>[2x]MRGSHHHHHHGLVPRGSMIRTMLQGKLHRVKVTHADLHYEG;>XCAIDQDFLDAAGILENEAIDIWNVTNGKRFSTYAIAAERGSRIISVNGAAAHCASVGDIVIIASFVTMPDEEARTWRP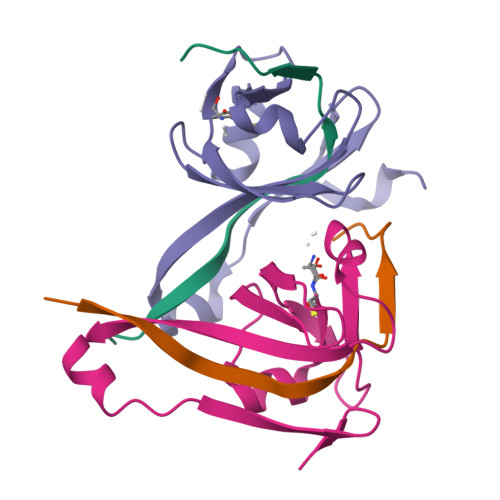NVAYFEGDNEMKRTAKAIPVQVA[2x]Naproxenoyl-CoA | C35 H48 N7 O18 P3 S | 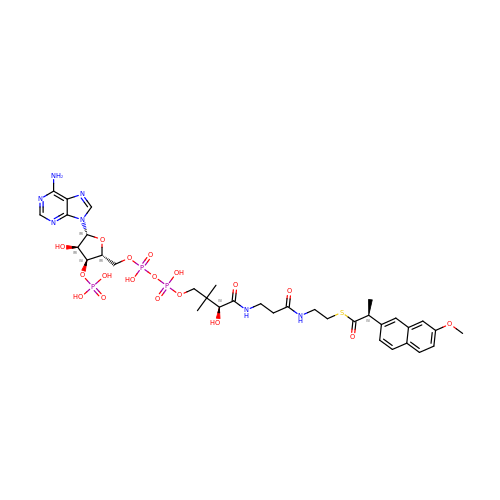SAHWFIOQEWXFSQ-PQXPHSRXSA-N> MKEALGLIETKGLVACIEAADAMCKAA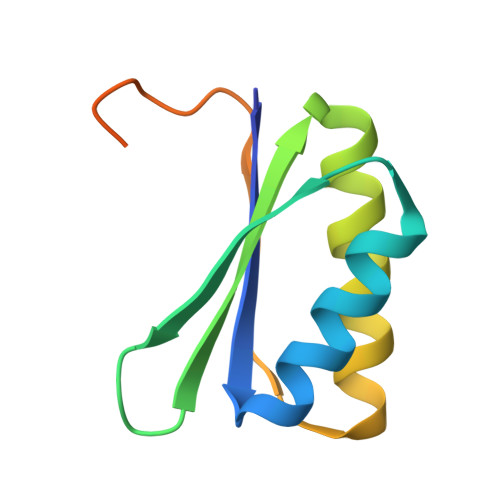NVELIGYENVGSGLVTAMVKGDVGAVNAAVDSGVEAAKRIGKVVSSRVIARPHNDIEKIAGSTKHKSLRPHNA> EAFEQQFLDVQNGQLRLNGEKVFMSGMNIAWQNYGRDFGNGQYDCCTGNALEDYIVRIKAEGGNSLRIWVHCDGGYTPEFDGNGYVVGTDAQNTMTSDLAQFLDVAYANNVLVFIVLWNGATTPTSRYRDLIYDDSKLQTYIDQALVPMVSALSGKVALGGWEVMNEPEGIVSAGVSDGNPCFDTQPLAGSGAGWADSIPMQRLQSFINKQTAAIKRADPKVIVTLGSWSERAQTDQFGWRNYYTDNCLIDAGGDSLGVIDFYQMHTYAWEGAYTSSSPLLVPNSQYNLDKPNNIGEFSQSGGDGRSITDQFDWAYTQGYCGAWSWQANG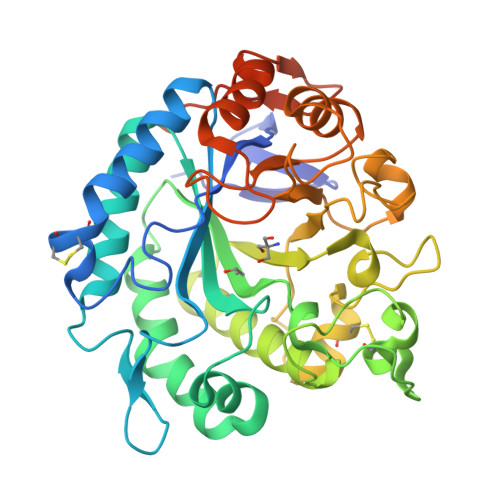GGDNADSFATQAQGLNHLRGRNDQNAGGRIDIILQLEQKLISEEDLNSAVDHHHHHH>GFEFTLMVVGESGLGKSTLINSLFLTDLYSPEYPGPSHRIKKTVQVEQSKVLIKEGGVQLLLTIVDTPGFGDAVDNSNCWQPVIDYIDSKFEDYLNAESRVNRRQMPDNRVQCCLYFIAPSGHGLKPLDIEFMKRLHEKVNIIPLIAKADTLTPEECQQFKKQIMKEIQEHKIKIYEFPETDDEEENKLVKKIKDRLPLAVVGSNTIIEVNGKRVRGRQYPWGVAEVENGEHCDFTILRNMLIRTHMQDLKDVTN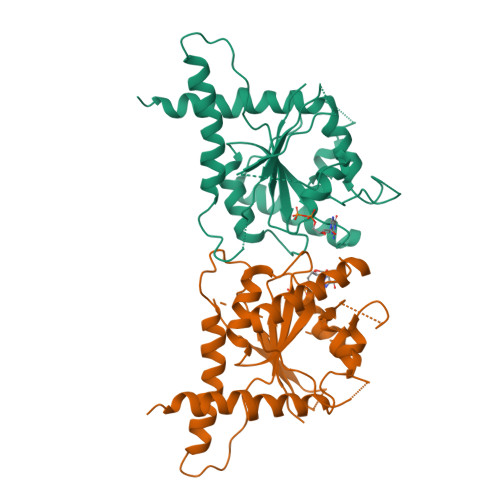NVHYENYRSRKLAAVT[2x]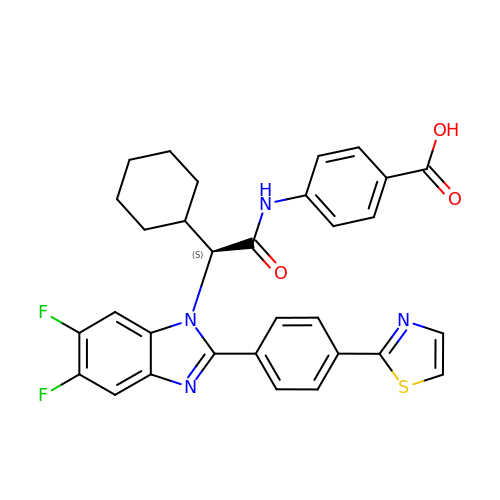4-{[(2S)-2-cyclohexyl-2-{5,6-difluoro-2-[4-(1,3-thiazol-2-yl)phenyl]-1H-benzimidazol-1-yl}acetyl]amino}benzoic acid | C31 H26 F2 N4 O3 S | DUGIQUVAQZHWSE-MHZLTWQESA-N> APVRSLNCRIWDVNQKTFYLRNNQLVAGYLQGPNVNLEEKFSMSFVQGEESNDKIPVALGLKEKNLYLSCVLKDD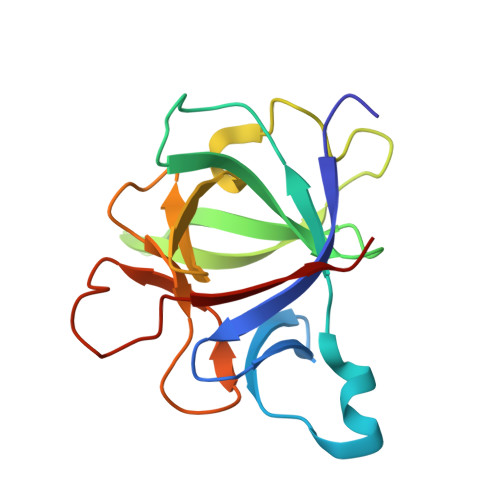KPTLQLESVDPKNYPKKKMEKRFVFNKIEINNKLEFESAQFPNWFLCTAMEADQPVSLTNMPDEGVMVTKFYMQFVSS Trehalose synthase (TS) catalyzes the reversible conversion of the inexpensive maltose into trehalose in the absence of any coenzyme. DrTS consists of a catalytic (β/α)8 barrel, subdomain B, a C-terminal β domain and two TS-unique subdomains (S7 and S8). Domain C and sub­domain S8 contribute to dimer formation, while subdomains B and S7 serve as a gateway for the opening and closing of the active site. In the present study, we have determined crystal structures of the wild type and the N253A mutant of TS from Deinococcus radiodurans (DrTS) that reveal a closed conformation for intramolecular isomerization.

The four or eight subunits in each asymmetric unit did not display significant differences, with root-mean-square deviations of 0.3–0.4 Å for all Cα atoms. The peak was assigned as a Tris from the crystallization solution, which contained 300 mM Tris–HCl, forming hydrogen bonds to Asp63, His106, Asp209, Glu251 and Arg398. In the wild-type structure, a similar Tris signal was also observed. Our present assay results indicated that the activity of DrTS is inhibited strongly by Tris, with a IC50 value of 4.88 mM in the presence of 50 mM maltose. Because of high structural homology, in particular similar active-site architectures and subdomain B orientations of TS to SH, AS and SI, we therefore conclude that the MsTS and MtTS structures may represent an open conformation of apo TS, while our DrTS–Tris complex represents a substrate-induced closed conformation for catalysis of the intramolecular isomerization. In particular, Arg148 forms salt bridges with Glu223 and Glu324, which form hydrogen bonds to Gln254 and Asn253, respectively. In addition, Asp153 forms two hydrogen bonds to Asn347. In DrTS, Ile150, Phe151 and Phe173 in subdomain B and His318, Asp319, Glu320 and Glu324 in S7 all constitute part of the active-site pocket. This means that interactions of the substrate with these residues would bring these two subdomains closer together to form a closed conformation.

>[8x]MVPTQAHPEWYKSAVFYELSVRTFQDGNGDGKGDFPGLTSRLDYLKNLGVDCLWLLPWFPSPLRDDGYDVADYRGIHPDLGTLDDFKVFLREAHARGLWVIGDLVTNHTSSDHPWFQAARRGPTLPDGSPNEYHDYYVWSDEGKEYADTRIIFTDTEVSNWTLDEQAGKYYWHRFFASQPDLNYDNPKVVEELHGAARFWLDLGLDGFRVDAVPYLIEREGTSCENLPETHEILKGFRAMVDREYPGRLLLAEANQWPEEVVEYFGTEAEPEFHMCFNFPVMPRLYMSLKREDTSSIREIMGRLPKIPSFGQWCIFLRNHDELTLEMVTDDERAFMYAAYAPDARMKINVGIRRRLAPLLDNDRRRIELLNTVLLALPGSPVLYYGDEIGMGDDLGLPDRNGVRTPMQWNAGTSGGFSTAQPSDCFFPPIQDPVYGFGRVNVQSQLQDPSSLLKWTARQLELRRAHPAFAHGDLTFIETGNPAILAFTRQYDGETLLIVSNFAGNAQAGLLDLAPFVGRAPVTLSGASPLPVVTGNGQYPVVMGKYDYYWLRLNSRVDKLAAALEHHHHHH> NLQTITLTKTHIDLYYMLVQMTDEFYPQLSAHGKQAVIHAPEDLTVSGDPDKLARVFNNILK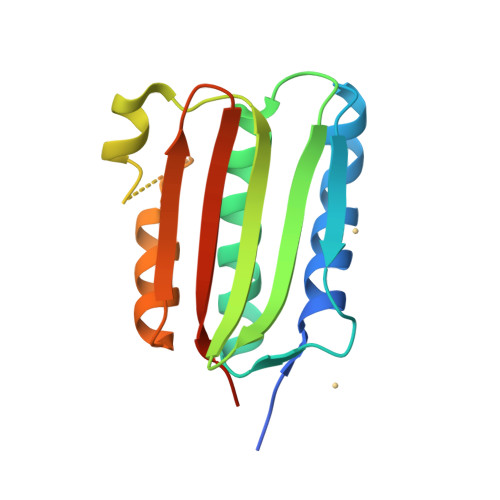NAAAYSEDNSIIDITAGLSGDVVSIEFKNTGSIPKDKLAAIFEKFYRLDNARSSDTGGAGLGLAIAKEIIVQHGGQIYAESNDNYTTFRVELPAMPDLVDKRRS>MSQQVEVVSFGPWSLDLSTRTLTREGQIVTLTTGEFAVLKALVQHPREPLTRDKLMNLARGREWGAME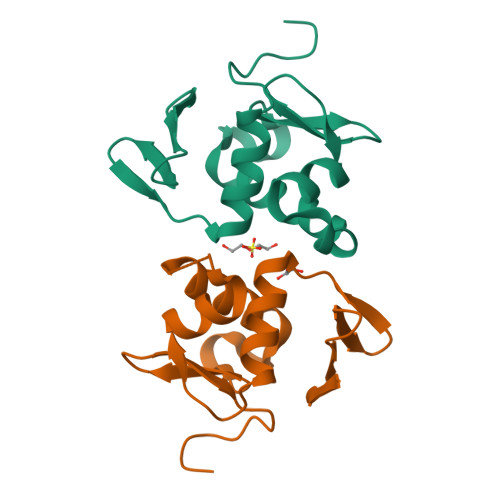RSIDVQVSRLRRLIEDNPARARYIQTVWGVGYVFVPDGAEHHHHHH[4x]>[6x]HHHHHHGSMTIPDVFPHLPLIAITRNPVFPRFIKIIEVKNKKLVELLRRKVRLAQPYVGVFLKRDDSNESDVVESLDEIYHTGTFAQIHEMQDLGDKLRMIVMGHRRVHISRQLEVEPEEPEAENKHKPRRKSKRGKKEAEDELSARHPAELAMEPTPELPAEVLMVEVENVVHEDFQVTEEVKALTAEIVKTIRDIIALNPLYRESVLQMMQAGQRVVDNPIYLSDMGAALTGAESHELQDVLEETNIPKRLYKALSLLKKEFELSKLQQRLGREVEEKIKQTHRKYLLQEQLKIIKKELGLEKDDKDAIEEKFRERLKELVVPKHVMDVVDEELSKLGLLDNHSSEFNVTRNYLDWLTSIPWGKYSNENLDLARAQAVLEEDHYGMEDVKKRILEFIAVSQLRGSTQGKILCFYGPPGVGKTSIARSIARALNREYFRFSVGGMTDVAEIKGHRRTYVGAMPGKIIQCL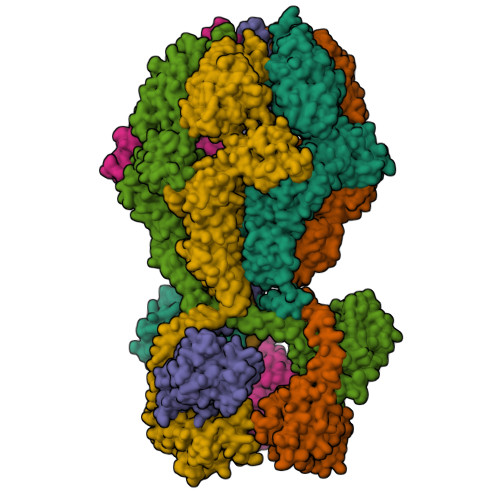KKTKTENPLILIDEVDKIGRGYQGDPSSALLELLDPEQNANFLDHYLDVPVDLSKVLFICTANVTDTIPEPLRDRMEMINVSGYVAQEKLAIAERYLVPQARALCGLDESKAKLSSDVLTLLIKQYCRESGVRNLQKQVEKVLRKSAYKIVSGEAESVEVTPENLQDFVGKPVFTVERMYDVTPPGVVMGLAWTAMGGSTLFVETSLRRPQDKDAKGDKDGSLEVTGQLGEVMKESARIAYTFARAFLMQHAPANDYLVTSHIHLHVPEGATPKDGPSAGCTIVTALLSLAMGRPVRQNLAMTGEVSLTGKILPVGGIKEKTIAAKRAGVTCIVLPAENKKDFYDLAAFITEGLEVHFVEHYREIFDIAFPDEQAEALAVER>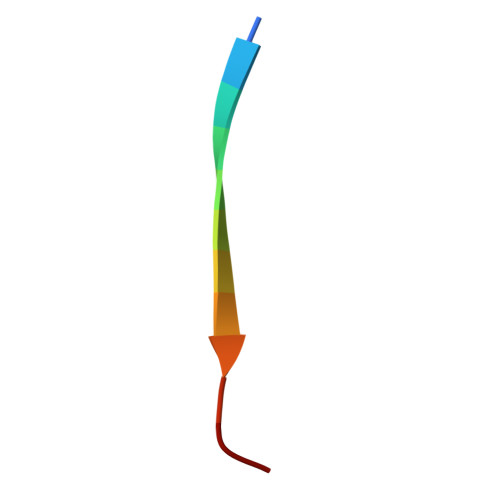 EPKLLLKINLKK4-(2-aminopropan-2-yl)-N'-[4-(cyclopropyloxy)-3-methoxybenzoyl]-6-(4-fluorophenyl)pyridine-2-carbohydrazide | C26 H27 F 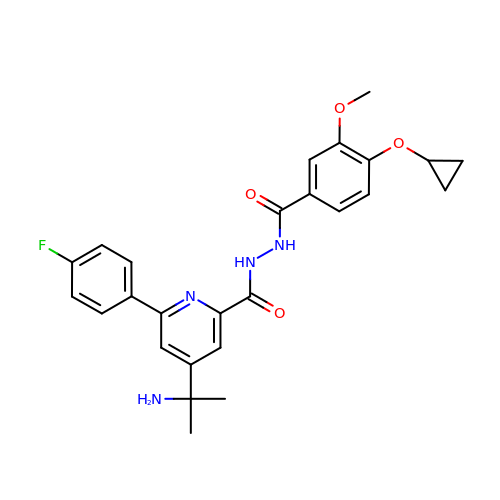N4 O4 | RLLFSRLPEMDZNU-UHFFFAOYSA-N>[14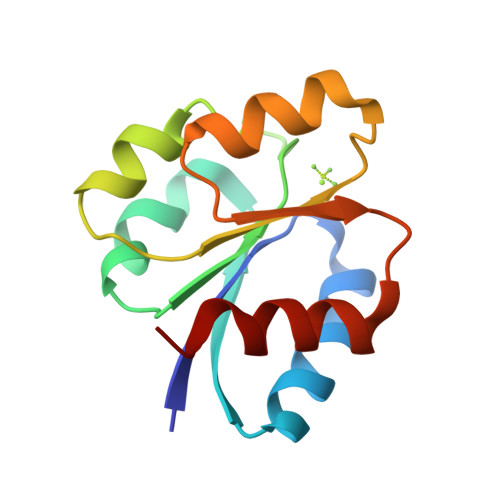x]MKQTLLLVEDDKNLADGLLVSLEQAGYECLHVERIADVEPQWKKADLVILDRQLPDGDSVQHLPEWKKIKDVPVILLTALVTVKDKVAGLDSGANDYLTKPFAEAELFARIRAQLRA> MDKLGENLNKALNKLKAAAFVDKKLIKEVIKDIQRALIQADVNVKLVLKMSKEIERRALEEKTPKGLSKKEHIIKIVYEELVKLLGEEAKKLELNPKKQNVILLVGIQGSGKTTTAAKLARYIQKRGLKPALIAADTYRPAAYEQLKQLAEKIHVPIYGDETRTKSPVDIVKEGMEKFKKADVLIIDTAGRHKEEKGLLEEMKQIKEITNPDEIILVIDGTIGQQAGIQAKAFKEAVGEIGSIIVTKLDGSAKGGGALSAVAETKAPIKF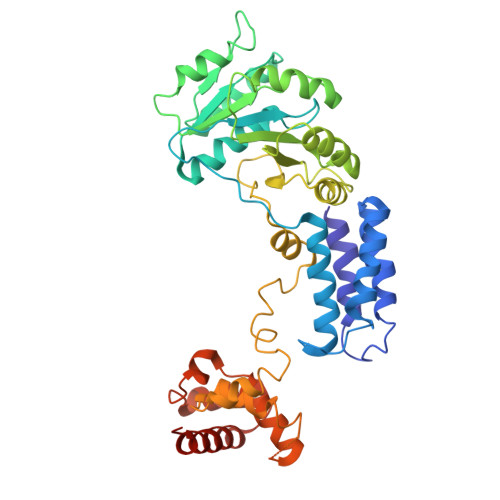IGIGEGIDDLEPFDPKKFISRLLGMGDLESLLEKAEDMVDEKTEESIDAIMRGKFTLNELMTQLEAIENMGSMKKILSMIPGFGGAMPKELSHLTEAKIKKYKVIISSMTKEERENPKIIKASRIRRIARGSGTTENDVREVLRYYETTKNAIDKLHHHHHH The KSHV latency-associated nuclear antigen (kLANA) and the MHV68 mLANA (orf73) protein are required for latent viral replication and persistence. We solved the X-ray crystal structure of the C-terminal DNA binding domains (CTD) of kLANA and MHV-68 mLANA. The C-terminal domain (CTD) of LANA forms dimers, which bind two adjacent DNA sequences, the LANA binding sites (LBS1 & LBS2) in a single TR. Importantly, kLANA and mLANA CTD dimers undergo higher order oligomerization.

During our crystallization trials, we obtained three different crystal forms of the kLANA CTD, all of which contained higher order oligomers. The monoclinic and orthorhombic crystals of the kLANA CTD contained pentameric rings of dimers, whereas the cubic crystals contained tetrameric rings of dimers. In all structures the oligomerization interfaces are formed by helices α1 and α3, and the interface comprises an area of approx. 500 Å2. In kLANA, the interface is mostly hydrophobic, whereas it has a more hydrophilic character in mLANA. The angles between two neighboring LANA dimers range from 0° for mLANA, 72° for the kLANA pentameric rings to 90° for the kLANA tetrameric ring. Moreover, both pentameric ring structures of kLANA dimers display ring puckering, where the interface between two dimers is oriented out of the ring plane. This provides direct crystallographic evidence that the interface between LANA dimers is generally compatible with a range of relative LANA dimer orientations. Due to the hinge-like character of the inter-dimer interface, in vivo native LANA oligomers might differ in shape from the closed ring structures or the linear chain observed in the respective crystals.

> GSGVRMRRVPVTHPKKPHPRYQQPPVPYRQIDDCPAKARPQHIFYRRFLGKDGRRDPKCQWKFAVIFWGNDPYGLKKLSQAFQFGGVKAGPVSCLPHPGPDQSPITYCVYVYCQNKDTSKKVQMARLAWEASHPLAGNLQSSIVKFKKPLPLTQPGENQG>[3x]MAHHHHHHMSKTPLSIAHPWHGPVLTRDDYESLCCYIEITPADSVKFELDKETGILKVDRPQKFSNFCPCLYGLLPKTYCGDLSGEYSGQQSNRENIKGDGDPLDICVLTEKNITQGNILLQARPIGGIRILDSEEADDKIIAVLEDDLVYGNIEDISECPGTVLDMIQHYFLTYKATPESLIQAKPAKIEIVGLYGKKEAQKVIRLAHEDYCNLFM

C. trachomatis inorganic pyrophosphatase (CtPPase) hydrolyzes inorganic pyrophosphate during metabolism. CtPPase is a small β-strand protein containing a core five-stranded oligonucleotide/oligosaccharide-binding (OB) fold. CtPPase has the prototypical family I pyrophosphatase (PPase) topology. Family 1 PPases are ubiquitous in all kingdoms of life. The overall topology of CtPPase resembles an open fist (or baseball mitt) with the substrate-binding cavity sitting in the palm, while β-strands form finger-like structures surrounding the active site.

The CtPPase structure was refined to 2.25 Å resolution in space group C2221 with three molecules in the asymmetric unit. Surface-area calculations by PISA suggest a hexamer as the most likely biological assembly. Electron density modeled as an Na atom was observed in the active site of each monomer. Despite the addition of pyrophosphate to the crystallization buffer, no density was observed for pyrophosphate or phosphate ions. Additionally, the flexible active-site loop is in the open conformation indicative of an apo structure without any substrate or product in the active site of CtPPase. Comparison of the CtPPase structure with those of MtPPase and BpPPase shows that the loop adjacent to the putative allosteric binding site has moved into the pocket compared with MtPPase and BpPPase, closing off this site. Inspection of the solvent-accessible surface of CtPPase reveals a medium-sized cleft that partially occupies the fragment-binding site of BpPPase. CtPPase has a pocket in proximity to the previously identified bacterial allosteric binding sites, suggesting the possibility of developing allosteric inhibitors of CtPPase.> ERSSNNFNYGAYHSLEAIYHEMDNIAADFPDLARRVKIG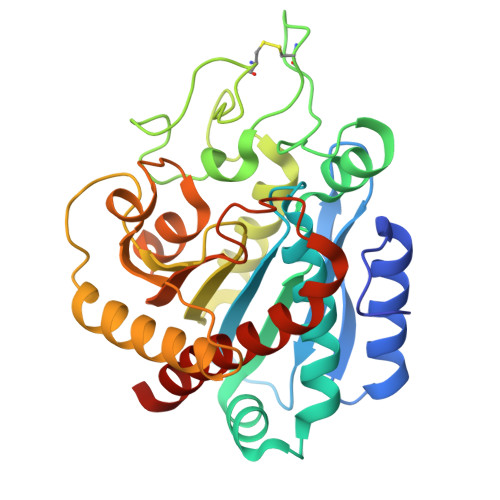HSFENRPMYVLKFSTGKGVRRPAVWLNAGIHSREWISQATAIWTARKIVSDYQRDPAITSILEKMDIFLLPVANPDGYVYTQTQNRLWRKTRSRNPGSSCIGADPNRNWNASFAGKGASDNPCSEVYHGPHANSEVEVKSVVDFIQKHGNFKGFIDLHSYSQLLMYPYGYSVKKAPDAEELDKVARLAAKALASVSGTEYQVGPTCTTVYPASGSSIDWAYDNGIKFAFTFELRDTGTYGFLLPANQIIPTAEETWLGLKTIMEHVRDNLY>ASLAA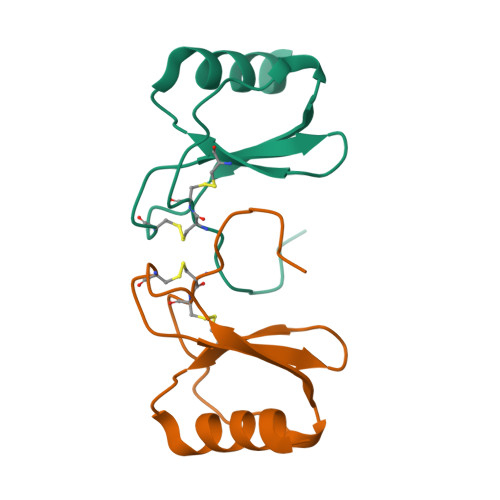DTATACCFSYTSRQIPQNFIADYFETSSQCSKPGVIFLTKRSRQVCADPSEEWVQKYVSDLELS[5x]> ADPQAGSLDLQIDEEQPAGTLIGDISAGLPAGTAAPLMYFISAQEGSGVGTDLAIDEHSGVVRTARVLDREQRDRYRFTAVTPDGATVEVTVRVADINDHAPAFPQARAALQVPEHTAFGTRYPLEPARDADAGRLGTQGYALSGDGAGETFRLETRPGPDGTPVPELVVTGELDRENRSHYMLQLEAYDGGSPPRR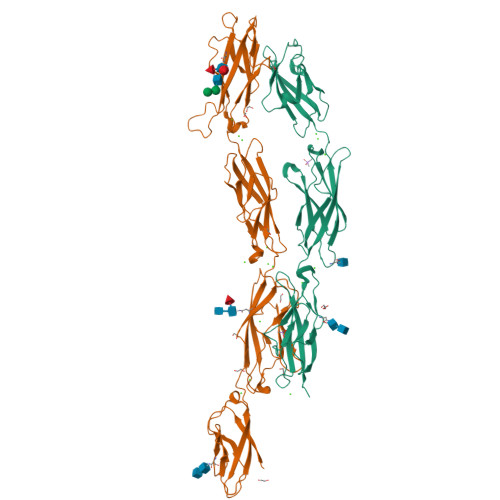AQALLDVTLLDINDHAPAFNQSRYHAVVSESLAPGSPVLQVFASDADAGVNGAVTYEINRRQSEGDGPFSIDAHTGLLQLERPLDFEQRRVHELVVQARDGGAHPELGSAFVTVHVRDAN;> MDLAPDRATGRPWLPLHTLSVSQLLRVFWLLSLLPGQAWVHGAEPRQVFQVLEEQPPGTLVGTIQTRPGFTYRLSESHALFAINSSTGALYTTSTIDRESLPSDVINLVVLSSAPTYPTEVRVLVRDLNDNAPVFPDPSIVVTFKEDSSSGRQVILDTATDSDIGSNGVDHRSYRIIRGNEAGRFRLDITLNPSGEGAFLHLVSKGGLDREVTPQYQLLVEVEDKGEPKRRGYLQVNVTVQDINDNPPVFGSSHYQAGVPEDAVVGSSVLQVAAADADEGTNADIRYRLQDEGTPFQMDPETGLITVREPLDFEARRQYSLTVQAMDRGVPSLTGRAEALIQLLDVNDNDPVVKFRYFPATSRYASVDENAQVGTVVALLTVTDADSPAANGNISVQILGGNEQRHFEVQSSKVPNLSLIKVASALDRERIPSYNLTVSVSDNYGAPPGAAVQARSSVASLVIFVND(2~{R})-2-(~{tert}-butylamino)-1-(3-chlorophenyl)propan-1-one 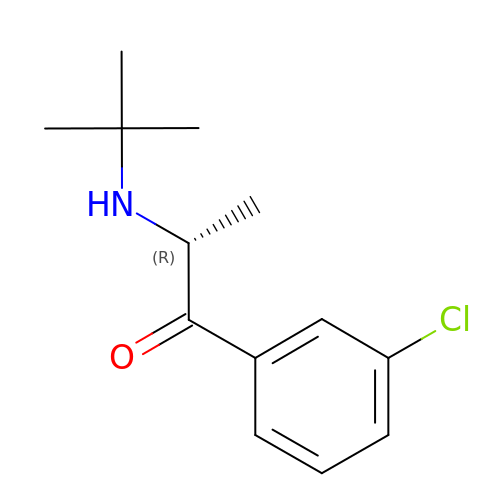| C13 H18 Cl N O | SNPPWIUOZRMYNY-SECBINFHSA-N>ISVSEKSKDRGSNTIGARLNRVEDKVTQLDQRLALITDMLHQLL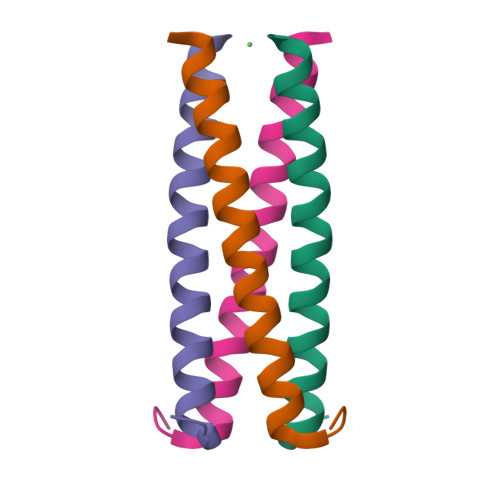SLHGG[2x]>DYKFWYTQPVPKINDEFNESVNEPFISDNKVEDVRKDEYKLPPGYSWYVCDVKDEKDRSEIYTLLTDNYVEDDDNIFRFNYSAEFLLWALTSPNYLKTWHIGVKYDASNKLIGFISAIPTDICIHKRTIKMAEVNFLCVHKTLRSKRLAPVLIKEITRRINLENIWQAIYTAGVYLPKPVSDARYYHRSINVKKLIEIGFSSLNSRLTMSRAIKLYRVEDTLNIKNMRLMKKKDVEGVHKLLGSYLEQFNLYAVFTKEEIAHWFLPIENVIYTYVNEENG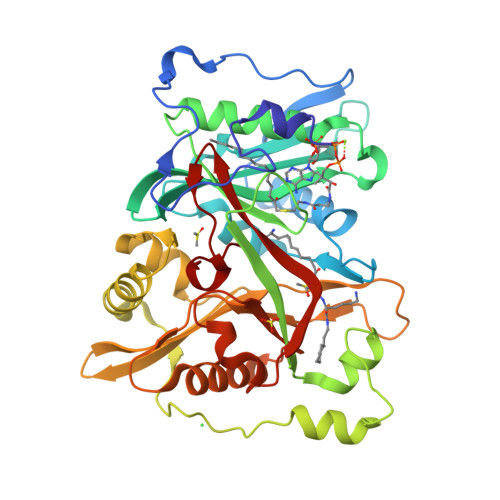KIKDMISFYSLPSQILGNDKYSTLNAAYSFYNVTTTATFKQLMQDAILLAKRNNFDVFNALEVMQNKSVFEDLKFGEGDGSLKYYLYNWKCASFAPAHVGIVLL[3x]> MRGSHHHHHHGSMRFAIVVTGPAYGTQQASSAFQFAQALIADGHELSSVFFYREGVYNANQLTSPASDEFDLVRAWQQLNAQHGVALNICVAAALRRG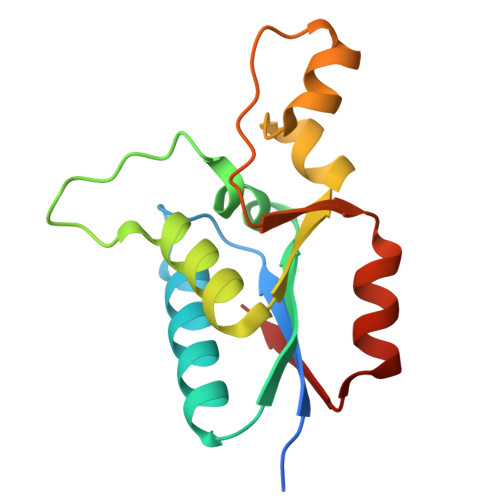VVDETEAGRLGLASSNLQQGFTLSGLGALAEASLTCDRVVQF> LLPLIKVLVVYPSEICFHHTVCRFTDFLQNYCRS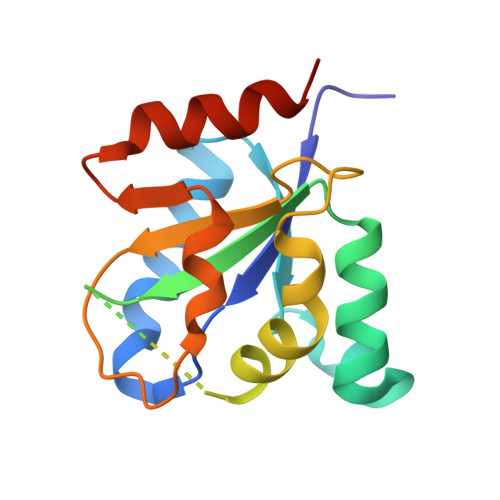EVILEAWQAAAIAEMGPVQWLTTQKQAADKVVFLLPSDVPTLCDSACGHNEGSARENSQDLFPLAFNLFCSDFSSQTHLHKYLVVYLGGADLKGDYNALSVCPQYHLMKDATAFHTELLKATQSMSVK> MTTYLEFIQQNEERDGVRFSWNVWPSSRLEATRMVVPVAALFTPLKERPDLPPIQYEPVLCSRTTCRAVLNPLCQVDYRAKLWACNFCYQRNQFPPSYAGISELNQPAELLPQFSSIEYVVLRGPQMPLIFLYVVDTCMEDEDLQALKESMQMSLSLLPPTALVGLITFGRMVQVHELGCEGISKSYVFRGTKDLSAKQLQEMLGLSKVPLTQATRGPQVQQPPPSNRFLQPVQKIDMNLTDLLGELQRDPWPVPQGKRPLRSSGVALSIAVGLLECTFPNTGARIMMFIGGPATQGPGMVVGDELKTPIRSWHDIDKDNAKYVKKGTKHFEALANRAATTGHVIDIYACALDQTGLLEMKCCPNLTGGYMVMGDSFNTSLFKQTFQRVFTKDMHGQFKMGFGGTLEIKTSREIKISGAIGPCVSLNSKGPCVSENEIGTGGTCQWKICGLSPTTTLAIYFEVVNQHNAPIPQ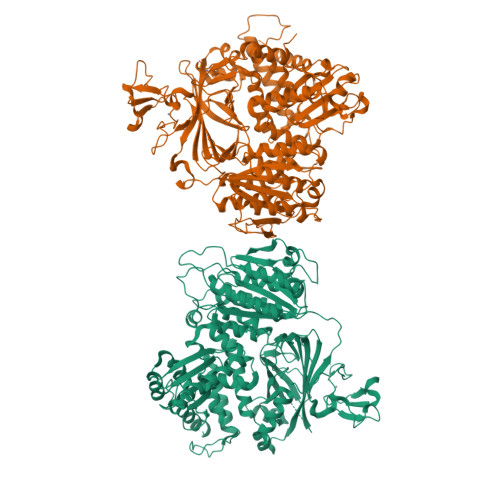GGRGAIQFVTQYQHSSGQRRIRVTTIARNWADAQTQIQNIAASFDQEAAAILMARLAIYRAETEEGPDVLRWLDRQLIRLCQKFGEYHKDDPSSFRFSETFSLYPQFMFHLRRSSFLQVFNNSPDESSYYRHHFMRQDLTQSLIMIQPILYAYSFSGPPEPVLLDSSSILADRILLMDTFFQILIYHGETIAQWRKSGYQDMPEYENFRHLLQAPVDDAQEILHSRFPMPRYIDTEHGGSQARFLLSKVNPSQTHNNMYAWGQESGAPILTDDVSLQVFMDHLKKLAVSSAA;> AMGSPIQVIENDRASRGGQVYATNTRGQIPPLVTTDCMIQDQGNASPRFIRCTTYCFPCTSDMAKQAQIPLAAVIKPFATIPSNESPLYLVNHGESGPVRCNRCKAYMCPFMQFIEGGRRYQCGFCNCVNDVPPFYFQHLDHIGRRLDHYEKPELSLGSYEYVATLDYCRKSKPPNPPAFIFMIDVSYSNIKNGLVKLICEELKTMLEKIPKEEQEETSAIRVGFITYNKVLHFFNVKSNLAQPQMMVVTDVGEVFVPLLDGFLVNYQESQSVIHNLLDQIPDMFADSNENETVFAPVIQAGMEALKAADCPGKLFIFHSSLPTAEAPGKLKNRDDKKLVNTDKEKILFQPQTNVYDSLAKDCVAHGCSVTLFLFPSQYVDVASLGLVPQLTGGTLYKYNNFQMHLDRQQFLNDLRNDIEKKIGFDAIMRVRTSTGFRATDFFGGILMNNTTDVEMAAIDCDKAVTVEFKHDDKLSEDSGALIQCAVLYTTISGQRRLRIHNLGLNCSSQLADLYKSCETDALINFFAKSAFKAVLHQPLKVIREILVNQTAHMLACYRKNCASPSAASQLILPDSMKVLPVYMNCLLKNCVLLSRPEISTDERAYQRQLVMTMGVADSQLFFYPQLLPIHTLDVKSTMLPAAVRCSESRLSEEGIFLLANGLHMFLWLGVSSPPELIQGIFNVPSFAHINTDMTLLPEVGNPYSQQLRMIMGIIQQKRPYSMKLTIVKQREQPEMVFRQFLVEDKGLYGGSSYVDFLCCVHKEICQLLN>[3x]MTIKNFTFFSPNSTEFPVGSNNDGKLYMMLTGMDYRTIRRKDWSSPLNTALNVQYTNTSIIAGGRYFELLNETVALKGDSVNYIHANIDLTQTANPVSLSAETANNSNGVDINNGSGVLKVCFDIVTTSGTGVT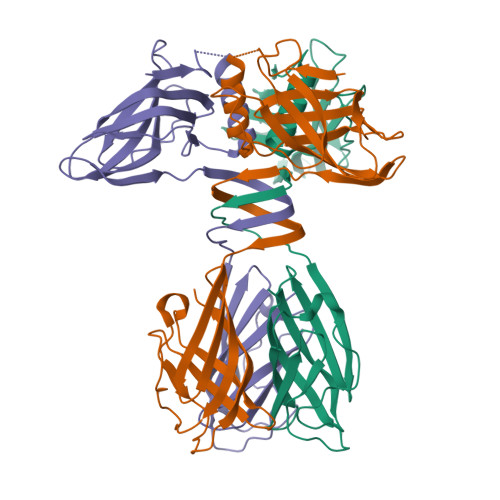STKPIVQTSTLDSISVNDMTVSGSIDVPVQTLTVEAGNGLQLQLTKKNNDLVIVRFFGSVSNIQKGWNMSGTWVDRPFRPAAVQSLVGHFAGRDTSFHIDINPNGSITWWGANIDKTPIATRGNGSYFIK(3R,4R)-N-(4-CHLOROPHENYL)-N'-[2-FLUORO-4-(2-OXOPYRIDIN-1(2H)-YL)PHENYL]-1-(2,2,2-TRIFLUOROETHYL)PYRROLIDINE-3,4-DICARBOXAMIDE 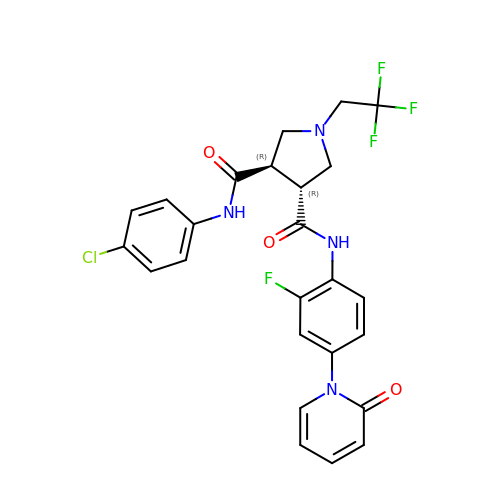| C25 H21 Cl F4 N4 O3 | TYMJFUUUNPEDQB-OALUTQOASA-N>[4x]GHMAEAFYEELKEKADIGEVAGDAIVSFQDVFFTTPRGRYDIDIYKNSIRLRGKTYEYKLQHRQIQRIVSLPKADDIHHLLVLAIEPPLRKGQTTYPF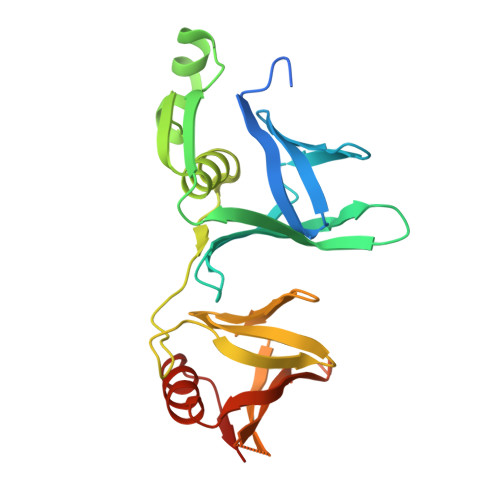LVLQFQKDEETEVQLNLEDEDYEENYKDKLKKQYDAKTHIVLSHVLKGLTDRRVIVPGEYKSKYDQCAVSCSFKANEGYLYPLDNAFFFLTKPTLYIPFSDVSMVNISRAGQTSTSSRTFDLEVVLRSNRGSTTFANISKEEQQLLEQFLKSKNLRVKNEDRE>MCNLVGRQRQEILELRREMEELSVSHDGVLIWKLSDYSRKLQEAKIRSNHEFF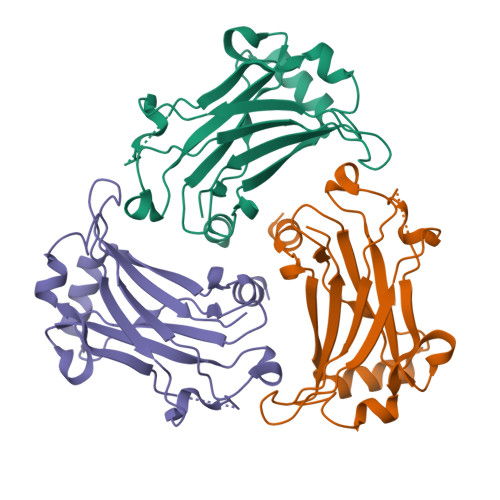SPPFYTHRYGYKLQVSAFLNGNGSGEGSHLSVYIRVLPGEYDSLLEWPFSYKVTFSIMDQSDPSLSKPQHITETFNPDPNWKNFQKPSSTRNSLDESTLGFGYPKFISHEEIKKRNYVRDNSVFIKASIEIPQKIMA[3x]>[4x]MKEHQGAYCTGTYRNLLAEYGYGEEAIQRRLDETWEQLFEGDEETRIYYPSGEDMGYMLDTGNLDVRT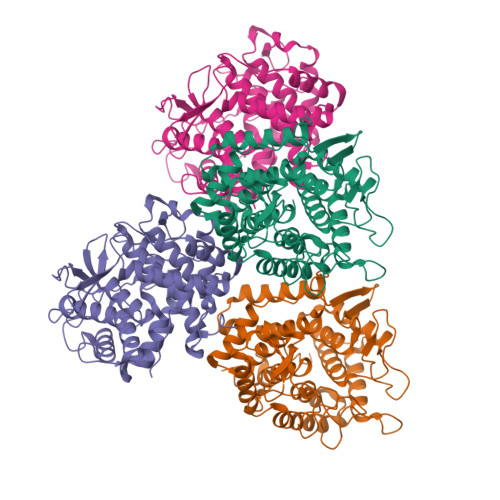EGMSYGMMMAVQYDRQDVFDRIWKWTVTYMYMTEGDNAGYFAWSCAPDGKRLSNGPAPDGEEYFALALLFASHRWGDREAPFNYGTQARDLLRTCLHKGEDGPGYPMWNPDNKLIKFVPNCEFSDPSYHLPHFYELFALWAYPEDRAFWKEAAEASRQYLHLACHPVTGLAPEYAYYDGTPNNERGYGHFFSDAYRVAANLGLDWEWFAADPWQREAVGKIQAFFADKEPEDYRRYTISGEPFEEPALHPVGLLATNAMASLAADGPQAKACVDLFWNTPVRTGKRRYYDNCLYLFALLALSGNYRIWMPRGEA>[4x]GAMAAPILKDVVAYVEVWSSNGTENYSKTFTTQLVDMG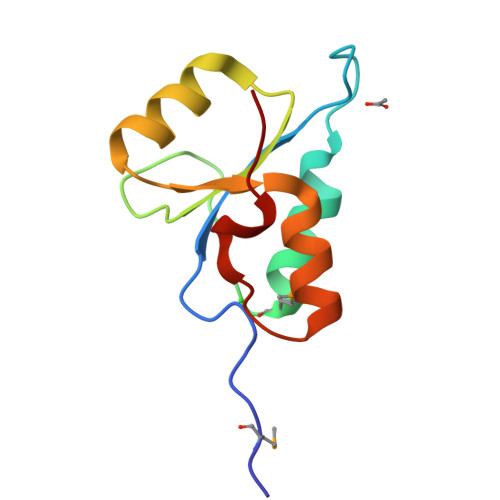AKVSKTFNKQVTHVIFKDGYQSTWDKAQKRGVKLVSVLWVEKCRTAGAHIDESLFPAAN(2S)-amino(carbamoylamino)ethanoic 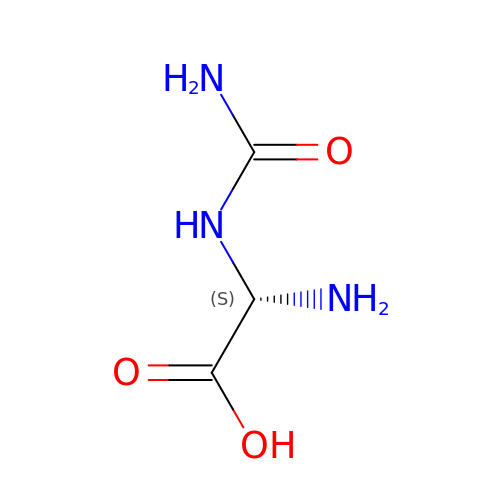acid | C3 H7 N3 O3 | VTFWFHCECSOPSX-SFOWXEAESA-N>[2x]KMPEEEQDSLAAFSRIEANITQYDPLLDNAGKSACTCICLKAAEMLLEASPDQVNAGLIDDILVEGVADYNRFKVGGVV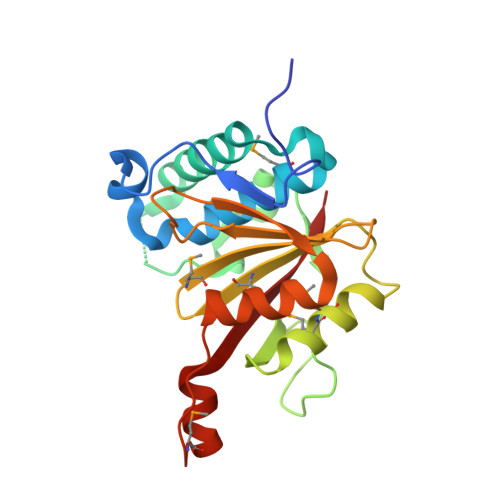EHTSVENYELNTFELKRLEFRDVDNPFSAEGNPYAGTLDSFAKMMEKASDSKDLPKPVALVMTKSNMTITIVIRPDGKYWLFDPHGTNGKGAYIESCNTDELIKKIKEIFPKTSYPGMTEDENLGFNSFEAYAVRR> MKKLYATLFSALVVGCAVCAGCTTKKVSSSAEVVDIIHKVNGYWQTNHPEHGRSFWDNAAYHTGNMEAYFLTNKPEYLEYSKGWAEHNEWKGAKSDHKANWKYSYGESNDYVLFGDYQICFQTYADLYNLEPDTHKIARAREVMEYQMSTPNNDYWWWADGLYMVMPVMTKLYNITKNPLYLEKLHEYLAYADSIMYDEEAGLYYRDGKYVYPKHKSVNGKKDFWARGDGWVLAGLAKVLKDLPETDKYRQEYIDRFRTLAKSVAACQQPEGYWTRSMLDAQHAPGPETSGTAFFTYGLQWGVNNGFLDSAHYQPVVEKAWKYLSTVALQPDGKIGYV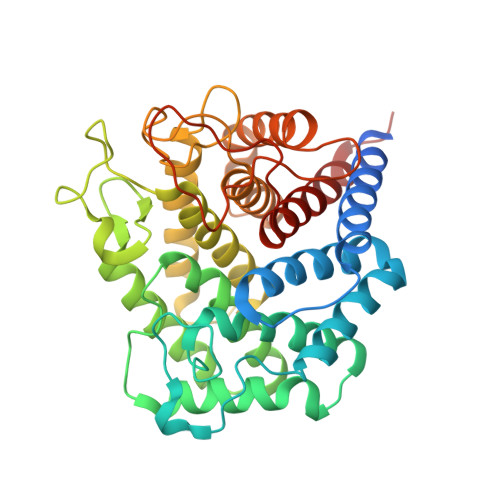QPIGEKAIPGQVVDANSTSNFGVGAFLLAACERVRYLESLIQH> MKIALINENSQASKNTIIYKELKAVSDEKGFEVFNYGMYGKEEESQLTY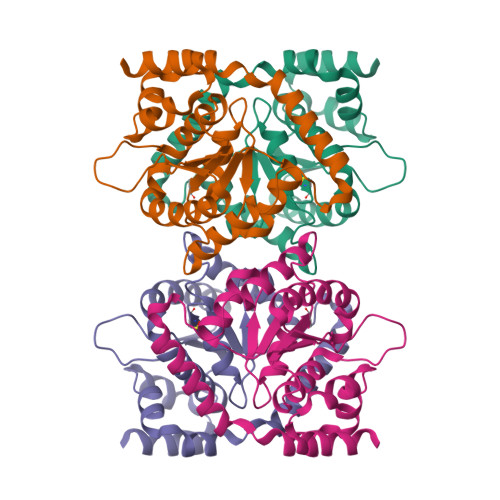VQNGLLTAILLNSGAADFVITGCGAGIGAMLACNSFPGVVCGFAADPVDAYLFSQVNGGNALSLPFAKGFGWGAELNLRYLFERLFEDEKGGGYPKERAVPEQRNARILSEIKQITYRDLLSVLKEIDQDFLKETISGEHFQEYFFANCQNQNIADYLKSVLDLEHHHHHH> DYWRAKHHPPKNN;> CNWTGVKCNRRGEVSEIQLKEKQLQGSLPVTSLRSLKSLTSLTLSSLQLTGVIPKEIGDFTELELLDLSDNSLSGDIPVEIFRLKKLKTLSLNTNNLEGHIPMEIGNLSGLVELMLFDNKLSGEIPRSIGELKNLQVLRAGGNKNLRGELPWEIGNCENLVMLGLAETSLSGKLPASIGNLKRVQTIAIYTSLLSGPIPDEIGYCTELQNLYLYQNSISGSIPTTIGGLKKLQSLLLWQNNLVGKIPTELGNCPELWLIDFSENLLTGTIPRSFGKLENLQELQLSVNQISGTIPEELTNCTKLTHLEIDNNLITGEIPSLMSNLRSLTMFFAWQNKLTGNIPQSLSQCRELQAIDLSYNSLSGSIPKEIFGLRNLTKLLLLSNDLSGFIPPDIGNCTNLYRLRLNGNRLAGSIPSEIGNLKNLNFVDISENRLVGSIPPAISGCESLEFLDLHTNSLSGSLLGT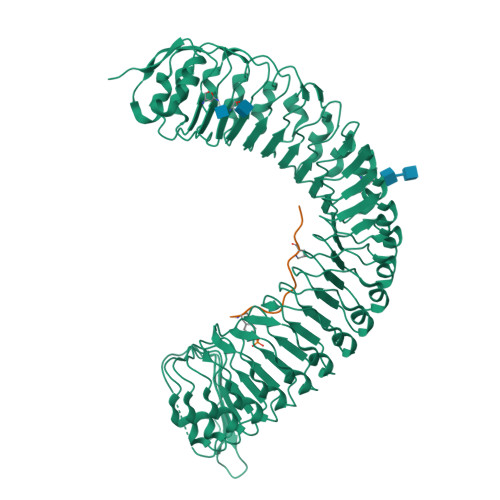TLPKSLKFIDFSDNALSSTLPPGIGLLTELTKLNLAKNRLSGEIPREISTCRSLQLLNLGENDFSGEIPDELGQIPSLAISLNLSCNRFVGEIPSRFSDLKNLGVLDVSHNQLTGNLNVLTDLQNLVSLNISYNDFSGDLPNTPFFRRLPLSDLASNRGLYISNAIST>[3x]MRGSHHHHHHGMASMAVSESQLKKMVSKYKYRDLTVRETVNVITLYKDLKPVLDSYVFNDGSSRELMNLTGTIPVPYRGNTYNIPICL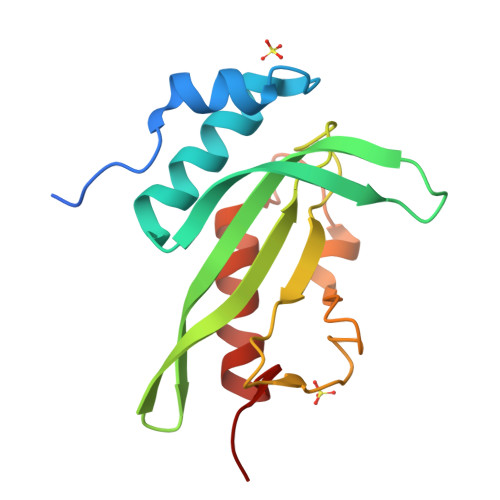WLLDTYPYNPPICFVKPTSSMTIKTGKHVDANGKIYLPYLHEWKHPQSDLLGLIQVMIVVFGDEPPVFSRP5-(hydroxymethyl)cytidine 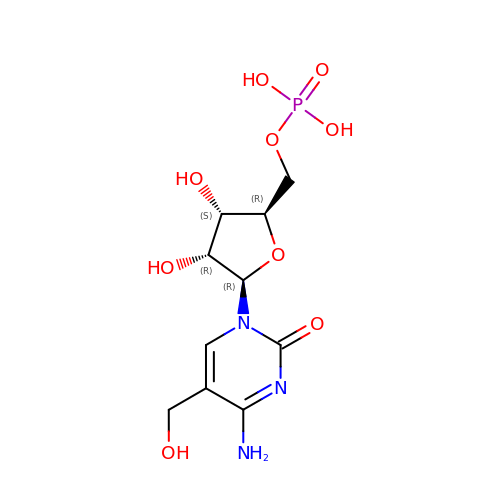5'-(dihydrogen phosphate) | C10 H16 N3 O9 P | KPUOHXMVCZBWQC-JXOAFFINSA-N Transcription factor (TF) IIIC, a six-subunit protein complex with a molecular weight (MW) of 624 kDa in humans, facilitates transcription of type 1 (5S ribosomal RNA) and type 2 [e.g., transfer RNAs (tRNAs)] RNA polymerase (Pol) III target genes. TFIIIC is composed of two subcomplexes, τA and τB, that bind two gene internal DNA motifs: A-box and B-box. τA binds the A-box with low affinity and is required to recruit TFIIIB to the promoter DNA. τB interacts with the B-box with high affinity and, therefore, is essential for target DNA recognition of type 2 genes. hTFIIIC consists of τA subunits TFIIIC35, TFIIIC63, and TFIIIC102 and τB subunits TFIIIC90, TFIIIC110, and TFIIIC220. TFIIIC220 forms an integral part of both τA and τB connecting the two subcomplexes via a ~550–amino acid residue flexible linker.

We determined cryo-EM structures of hTFIIIC alone and in complex with the TRR-TCT3-2 tRNA gene. In both cases, we obtained two distinct sets of particles for human τA and τB. Hence, TFIIIC90-TFIIIC110 form, with the help of the TFIIIC220 WH1 domain and the C-terminal zinc fingers in TFIIIC90, a stable scaffold, which stabilizes the WH2 and WH4 domains. TFIIIC110 and TFIIIC90 along with the TFIIIC220-WH1, WH2, and WH4 domains form a rigid τB scaffold, while WH3 and eWH domains remain flexible. WH2 and WH4 of TFIIIC220 are an integral part of the rigid τB-core, formed by TFIIIC90-TFIIIC110 and the TFIIIC220-WH1 domain, and their conformation does not change upon DNA binding, suggesting that they provide the platform for initial DNA recognition. TFIIIC dimerization is likely to be concentration dependent because our MP measurements did not show clear indications for dimer formation at nanomolar concentrations. The observation that TFIIIC dimerizes under cryo-EM conditions should be treated with care because we were unable to evaluate TFIIIC110 dimerization in solution due to a limited amount of protein sample.

>[2x]MDALESLLDEVALEGLDGLCLPALWSRLETRVPPFPLPLEPCTQEFLWRALATHPGISFYEEPRERPDLQLQDRYEEIDLETGILESRRDPVALEDVYPIHMILENKDGIQGSCRYFKERKNITNDIRTKSLQPRCTMVEAFDRWGKKLIIVASQAMRYRALIGQEGDPDLKLPDFSYCILERLGRSRWQGELQRDLHTTAFKVDAGKLHYHRKILNKNGLITMQSHVIRLPTGAQQHSILLLLNRFHVDRRSKYDILMEKLSVMLSTRTNHIETLGKLREELGLCERTFKRLYQYMLNAGLAKVVSLRLQEIHPECGPCKTKKGTDVMVRCLKLLKEFKRNDHDDDEDEEVISKTVPPVDIVFERDMLTQTYDLIERRGTKGISQAEIRVAMNVGKLEARMLCRLLQRFKVVKGFMEDEGRQRTTKYISCVFAEESDLSRQYQREKARSELLTTVSLASMQEESLLPEGEDTFLSESDSEEERSSSKRRGRGSQKDTRASANLRPKTQPHHSTPTKGGWKVVNLHPLKKQPPSFPGAAEERACQSLASRDSLLDTSSVSEPNVSFVSHCADSNSGDIAVIEEVRMENPKESSSSLKTGRHSSGQDKPHETYRLLKRRNLIIEAVTNLRLIESLFTIQKMIMDQEKQEGVSTKCCKKSIVRLVRNLSEEGLLRLYRTTVIQDGIKKKVDLVVHPSMDQNDPLVRSAIEQVRFRISNSSTANRVKTSQPPVPQGEAEEDSQGKEGPSGSGDSQLSASSRSESGRMKKSDNKMGITPLRNYHPIVVPGLGRSLGFLPKMPRLRVVHMFLWYLIYGHPASNTVEKPSFISERRTIKQESGRAGVRPSSSGSAWEACSEAPSKGSQDGVTWEAEVELATETVYVDDASWMRYIPPIPVHRDFGFGWALVSDILLCLPLSIFIQIVQVSYKVDNLEEFLNDPLKKHTLIRFLPRPIRQQLLYKRRYIFSVVENLQRLCYMGLLQFGPTEKFQDKDQVFIFLKKNAVIVDTTICDPHYNLARSSRPFERRLYVLNSMQDVENYWFDLQCVCLNTPLGVVRCPRVRKNSSTDQGSDEEGSLQKEQESAMDKHNLERKCAMLEYTTGSREVVDEGLIPGDGLGAAGLDSSFYGHLKRNWIWTSYIINQAKKENTAAENGLTVRLQTFLSKRPMPLSARGNSRLNIWGEARVGSELCAGWEEQFEVDREPSLDRNRRVRGGKSQKRKRLKKDPGKKIKRKKKGEFPGEKSKRLRYHDEADQSALQRMTRLRVTWSMQEDGLLVLCRIASNVLNTKVKGPFVTWQVVRDILHATFEESLDKTSHSVGRRARYIVKNPQAYLNYKVCLAEVYQDKALVGDFMNRRGDYDDPKVCANEFKEFVEKLKEKFSSALRNSNLEIPDTLQELFARYRVLAIGDEKDQTRKEDELNSVDDIHFLVLQNLIQSTLALSDSQMKSYQSFQTFRLYREYKDHVLVKAFMECQKRSLVNRRRVNHTLGPKKNRALPFVPMSYQLSQTYYRIFTWRFPSTICTESFQFLDRMRAAGKLDQPDRFSFKDQDNNEPTNDMVAFSLDGPGGNCVAVLTLFSLGLISVDVRIPEQIIVVDSSMVENEVIKSLGKDGSLEDDEDEEDDLDEGVGGKRRSMEVKPAQASHTNYLLMRGYYSPGIVSTRNLNPNDSIVVNSCQMKFQLRCTPVPARLRPAAAPLEELTMGTSCLPDTFTKLINPQENTCSLEEFVLQLELSGYSPEDLTAALEILEAIIATGCFGIDKEELRRRFSALEKAGGGRTRTFADCIQALLEQHQVLEVGGNTARLVAMGSAWPWLLHSVRLKDREDADIQREDPQARPLEGSSSEDSPPEGQAPPSHSPRGTKRRASWASENGETDAEGTQMTPAKRPALQDSNLAPSLGPGAEDGAEAQAPSPPPALEDTAAAGAAQEDQEGVGEFSSPGQEQLSGQAQPPEGSEDPRGFTESFGAANISQAARERDCESVCFIGRPWRVVDGHLNLPVCKGMMEAMLYHIMTRPGIPESSLLRHYQGVLQPVAVLELLQGLESLGCIRKRWLRKPRPVSLFSTPVVEEVEVPSSLDESPMAFYEPTLDCTLRLGRVFPHEVNWNKWIHLGGGSGGGSGGSLEVLFQGPGSGSDYKDDDDKGDYKDDDDKGDYKDDDDK;>MNTADQARVGPADDGPAPSGEEEGEGGGEAGGKEPAADAAPGPSAAFRLMVTRREPAVKLQYAVSGLEPLAWSEDHRVSVSTARSIAVLELICDVHNPGQDLVIHRTSVPAPLNSCLLKVGSKTEVAECKEKFAASKDPTVSQTFMLDRVFNPEGKALPPMRGFKYTSWSPMGCDANGRCLLAALTMDNRLTIQANLNRLQWVQLVDLTEIYGERLYETSYRLSKNEAPEGNLGDFAEFQRRHSMQTPVRMEWSGICTTQQVKHNNECRDVGSVLLAVLFENGNIAVWQFQLPFVGKESISSCNTIESGITSPSVLFWWEYEHNNRKMSGLIVGSAFGPIKILPVNLKAVKGYFTLRQPVILWKEMDQLPVHSIKCVPLYHPYQKCSCSLVVAARGSYVFWCLLLISKAGLNVHNSHVTGLHSLPIVSMTADKQNGTVYTCSSDGKVRQLIPIFTDVALKFEHQLIKLSDVFGSVRTHGIAVSPCGAYLAIITTEGMINGLHPVNKNYQVQFVTLKTFEEAAAQLLESSVQNLFKQVDLIDLVRWKILKDKHIPQFLQEALEKKIESSGVTYFWRFKLFLLRILYQSMQKTPSEALWKPTHEDSKILLVDSPGMGNADDEQQEEGTSSKQVVKQGLQERSKEGDVEEPTDDSLPTTGDAGGREPMEEKLLEIQGKIEAVEMHLTREHMKRVLGEVYLHTWITENTSIPTRGLCNFLMSDEEYDDRTARVLIGHISKKMNKQTFPEHCSLCKEILPFTDRKQAVCSNGHIWLRCFLTYQSCQSLIYRRCLLHDSIARHPAPEDPDWIKRLLQSPCPFCDSPVF[2x];>[2x]MHHHHHHENLYFQGMDTCGVGYVALGEAGPVGNMTVVDSPGQEVLNQLDVKTSSEMTSAEASVEMSLPTPLPGFEDSPDQRRLPPEQESLSRLEQPDLSSEMSKVSKPRASKPGRKRGGRTRKGPKRPQQPNPPSAPLVPGLLDQSNPLSTPMPKKRGRKSKAELLLLKLSKDLDRPESQSPKRPPEDFETPSGERPRRRAAQVALLYLQELAEELSTALPAPVSCPEGPKVSSPTKPKKIRQPAACPGGEEVDGAPRDEDFFLQVEAEDVEESEGPSESSSEPEPVVPRSTPRGSTSGKQKPHCRGMAPNGLPNHIMAPVWKCLHLTKDFREQKHSYWEFAEWIPLAWKWHLLSELEAAPYLPQEEKSPLFSVQREGLPEDGTLYRINRFSSITAHPERWDVSFFTGGPLWALDWCPVPEGAGASQYVALFSSPDMNETHPLSQLHSGPGLLQLWGLGTLQQESCPGNRAHFVYGIACDNGCIWDLKFCPSGAWELPGTPRKAPLLPRLGLLALACSDGKVLLFSLPHPEALLAQQPPDAVKPAIYKVQCVATLQVGSMQATDPSECGQCLSLAWMPTRPHQHLAAGYYNGMVVFWNLPTNSPLQRIRLSDGSLKLYPFQCFLAHDQAVRTLQWCKANSHFLVSAGSDRKIKFWDLRRPYEPINSIKRFLSTELAWLLPYNGVTVAQDNCYASYGLCGIHYIDAGYLGFKAYFTAPRKGTVWSLSGSDWLGTIAAGDISGELIAAILPDMALNPINVKRPVERRFPIYKADLIPYQDSPEGPDHSSASSGVPNPPKARTYTETVNHHYLLFQDTDLGSFHDLLRREPMLRMQEGEGHSQLCLDRLQLEAIHKVRFSPNLDSYGWLVSGGQSGLVRIHFVRGLASPLGHRMQLESRAHFNAMFQPSSPTRRPGFSPTSHRLLPTP> IVGGYTCQENSVPYQVSLNSGYHFCGGSLINDQWVVSAAHCYKSRIQVRLGEHNINVLEGNEQFVNAAKIIKHPNFDRKTLNNDIMLIKLSSPVKLNARVATVALPSSCAPAGTQCLISGWGNTLSSGVNEPDLLQCLDAPLLPQADCEASYPGKITDNMVCVGFLEGGKDSC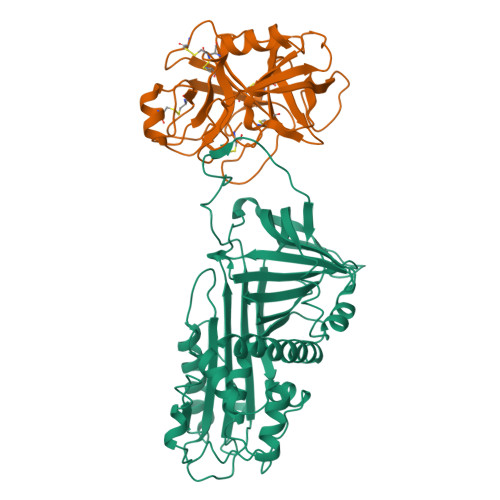QGDAGGPVVCNGELQGIVSWGYGCALPDNPGVYTKVCNYVDWIQDTIAAN;> MAGETDLQKILRESNDQFTAQMFSEVVKANPGQNVVLSAFSVLPPLGQLALASVGESHDELLRALALPNDNVTKDVFADLNRGVRAVKGVDLKMASKIYVAKGLELNDDFAAVSRDVFGSEVQNVDFVKSVEAAGAINKWVEDQTNNRIKNLVDPDALDETTRSVLVNAIYFKGSWKDKFVKERTMDRDFHVSKDKTIKVPTMIGKKDVRYADVPELDAKMIEMSYEGDQASMIIILPNQVDGITALEQKLKDPKALSRAEERLYNTEVEITLPKFKIETTTDLKEVLSNMNIKKLFTPGAARLENLLKTKESLTVDAAIQKAFIEVNEEGAEAAAANAFGIVPKSLILYPEVHIDRPFYFELKIDGIPMFNGKVIEP>[4x]ASWSH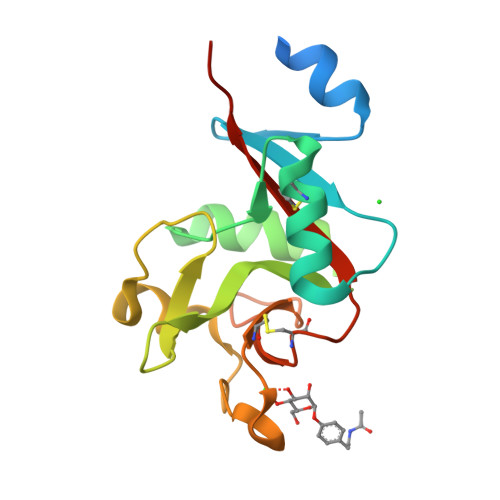PQFEKIEGRMQNDILQVVSQGWKYFKGNFYYFSLIPKTWYSAEQFCVSRNSHLTSVTSESEQEFLYKTAGGLIYWIGLTKAGMEGDWSWVDDTPFNKVQSARFWIPGEPNNAGNNEHCGNIKAPSLQAWNDAPCDKTFLFICKRPYVPSEP;> SW>[2x]VGLTDLTFRLLRESFADAVSWVAKNLPARPAVPVLSGVLLTGSDNGLTISGFDYEVSAEAQVGAEIVSPGSVLVSGRLLSDITRALPNKPVDVHVEGNRVALTCGNARFSLPTMPVEDYPTLPTLPEETGLLPAELFAEAISQVAIAAGRDDTLPMLTGIRVEILGETVVLAATDRFRLA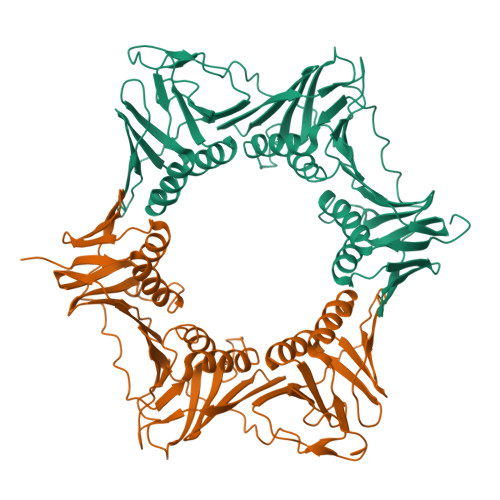VRELKWSASSPDIEAAVLVPAKTLAEAAKAGIGGSDVRLSLGTGPGVGKDGLLGISGNGKRSTTRLLDAEFPKFRQLLPTEHTAVATMDVAELIEAIKLVALVADRGAQVRMEFADGSVRLSAGADDVGRAEEDLVVDYAGEPLTIAFNPTYLTDGLSSLRSERVSFGFTTAGKPALLRPVSGDDRPVAGLNGNGPFPAVSTDYVYLLMPVRLPG>[2x]MVLYFIGLGLYDERDITVKGLEIAKKCDYVFAEFYTSLMAGTTLGRIQKLIGKEIRVLSREDVELNFENIVLPLAKENDVAFLTPGDPLVATTHAELRIRAKRAGVESYVIHAPSIYSAVGITGLHIYKFGKSATVAYPEGNWFPTSMYDVIKENAERGLHTLLFLDIKAEKRMYMTANEAMELLL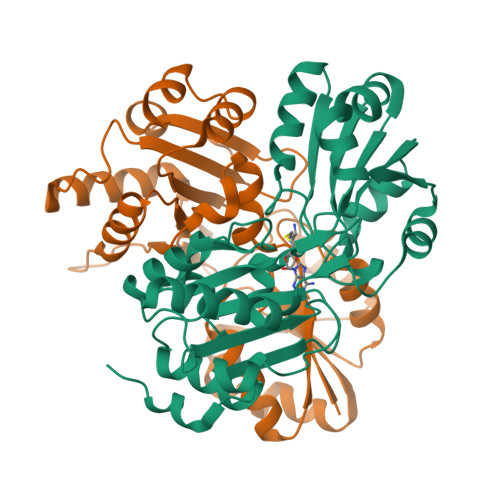KVEDMKKGGVFTDDTLVVVLARAGSLNPTIRAGYVKDLIREDFGDPPHILIVPGKLHIVEAEYLVEIAGAPREILRVNV>[2x]MLSTVFRRTMATGRHFIAVCQMTSDNDLEKNFQAAKNMIERAGEKKCEMVFLPECFDFIGLNKNEQIDLAMATDCEYMEKYRELARKHNIWLSLGGLHHKDPSDAAHPWNTHLIIDSDGVTRAEYNKLHLFDLEIPG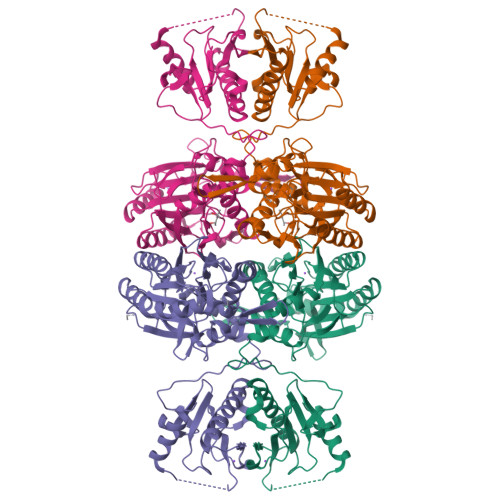KVRLMESEFSKAGTEMIPPVDTPIGRLGLSICYDVRFPELSLWNRKRGAQLLSFPSAFTLNTGLAHWETLLRARAIENQCYVVAAAQTGAHNPKRQSYGHSMVVDPWGAVVAQCSERVDMCFAEIDLSYVDTLREMQPVFSHRRSDLYTLHINEKSSETGGLKFARFNIPADHIFYSTPHSFVFVNLKPVTDGHVLVSPKRVVPRLTDLTDAETADLFIVAKKVQAMLEKHHNVTSTTICVQDGKDAGQTVPHVHIHILPRRAGDFGDNEIYQKLASHDKEPERKPRSNEQMAEEAVVYRNLM>MAHHHHHHMDSSRLSGNKSTYTDLQTTSEQFLFSSESVCSGHPDKLCDQISDAILDACLEQDPESFVACETCTKTGFIMVFGEITTKANVNYERVVRETVKEIGYDSEEKGLDYKTMDVIIKLEQQSNQAAGCVHVDKNVEDIGAGDQGMMFGYATNETKELMPLTHVLATSITRELDYIRMKGVSSRVGWLRPDGKAQVTVEYNCKHGVLIPKRIHTILVSVQHDENIENEEIREFVLENVIKKVCPSDLMDKETRILINPSGRFTIGGPAADAGLTGRKIIVDTYGGWGAHGGGAFSGKDATKVDRSGAYMARLVAKSIVFSGLCSRCLVQVSYGAGIARPLSLYINTFGTAKDGYNDTKLLEIVNK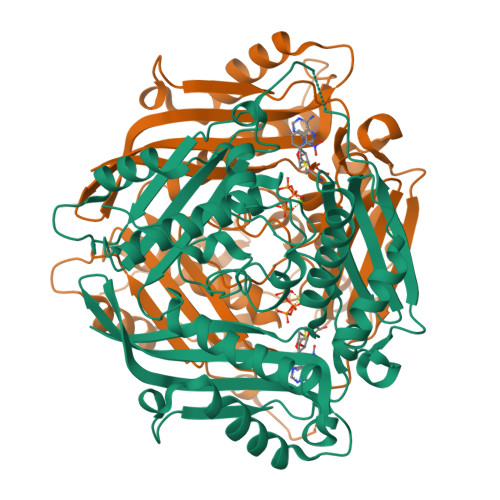VFDFRPGILIKQLNLKSPIFKKTSSGGHFGRSEKEFLWEKPIILQ[2x]>[4x]MHHHHHHAMGNKIVFVEDDPEVGTLIAAYLGKHDMDVVVEPRGDRAEEVIAREKPDLVLLDIMLPGKDGMTLCRDLRGQWQGPIVLLTSLDSDMNHILSLEMGASDYILKTTPPAVLLARLRLHLRQH

The RstB/RstA system is a ubiquitous TCS composed of the membrane-associated histidine kinase RstB and its cognate response regulator RstA. K. pneumoniae RstA (kpRstA) contains an N-terminal receiver domain (RD, residues 1–119) and a C-terminal DNA-binding domain (DBD, residues 131–236), with an overall sequence identity of 79% compared to RstA from E. coli and S. enterica serovar Typhimurium. As a member of the OmpR/PhoB subfamily, phosphorylation of the conserved Asp in the RD is believed to result in dimerization of the domain through a conserved α4–β5–α5 region, accompanied by the binding of the DBD to cognate sequences in the promoter region of RstA-regulated genes. Genomic systematic evolution of ligands by exponential enrichment (SELEX) experiments in E. coli have shown that RstA binds to the consensus sequence TACATNTNGTTACA with tandem TACA recognition sites.

The structure of kpRstA RD in the presence of BeF3− was solved to a resolution of 3.2 Å. Similar to the structure reported for TorR RD, four kpRstA RD molecules, which correspond to two dimers, were found in the asymmetric unit. The two dimers within the asymmetric unit had similar structures as revealed by structural alignment, with an rmsd of 0.47 Å over 117 Cα. Structural analyses revealed that the overall structure of kpRstA RD has the traditional (βα)5 fold of RR regulatory domains that consists of a central five-stranded parallel β-sheet surrounded by five-helices. In kpRstA RD, the BeF3− molecule is non-covalently bound to Asp52 within the phosphorylation site, and forms a hydrogen bond with the side-chain of Thr79, a salt bridge to Lys101, and van der Waals contacts with the backbone nitrogen atoms of Ile53, Met54 and Ser80. The interactions found in the phosphorylation site of kpRstA RD are analogous to those of other structures of active RRs from different subfamilies, underscoring the conserved nature of the phosphorylation site environment. The dimer interface of kpRstA RD has a buried surface area of 689.5 Å2 as calculated with PISA. Two conserved intermolecular salt bridges are formed between Asp97 (β5)–Arg111 (α5) at the center and Glu92 (α4)–Arg113 (α5) at the outer sides of the interface. Additionally, six hydrophobic residues (Ile88, Leu91, Ala106, Val107, Ala110 and Leu114) cluster together to form an extensive hydrophobic patch that holds together the α4 and α5 helices between adjacent molecules. Incidentally, the RD of kpRstA contains an extensive hydrophobic patch at the α4–β5–α5 region, which forms the dimer interface in the active form.>MGKGEGEVAGCKAAARLGVEGVFVEECFDGSYCRNLERIGYLRKGRLEPLEAAYQASRGMLCMGETRGWAAAVEVIAGLGLSLDTALVYFDLRRKGRKPLVGVRRGTLVYEHGGRVYEVLVLSEGYPLKIGSLVEWSRGASMDNHSPIVAIVDRTGLITYYEARAVRSIQ[6x];>[6x]MGDRCA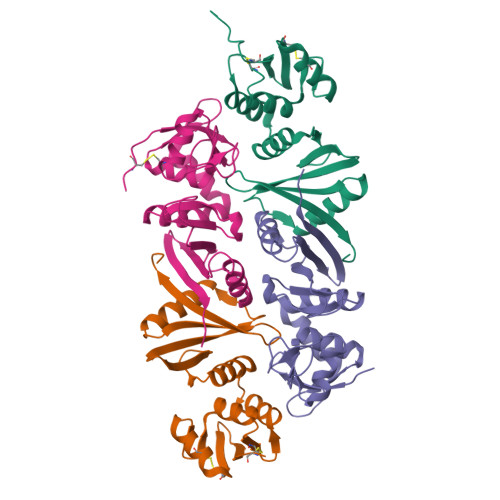PIKASGVLIGDSVLVTDVEQARSLYSCGYYGQPLDVEKPRGADFEGPLRLSLIESLYLAEKGVLEVAKPDGSSVGVEDLRTAVRGNPRFSMLYNIYRDLRERGFVVRSGLKFGSDFAVYRLGPGIDHAPFIVHAYSPEDNIDPVEIVRAGRLSHSVRKKFVFAVTRGGDVSYLMIDWFRP> VVGGTEAQRNSWPSQISLQYRSGSSWAHTCGGTLIRQNWVMTAAHCVDRELTFRVVVGEHNLNQNNGTEQYVGVQKIVVHPYWNTDDVAAGYDIALLRLAQSVTLNSYVQLG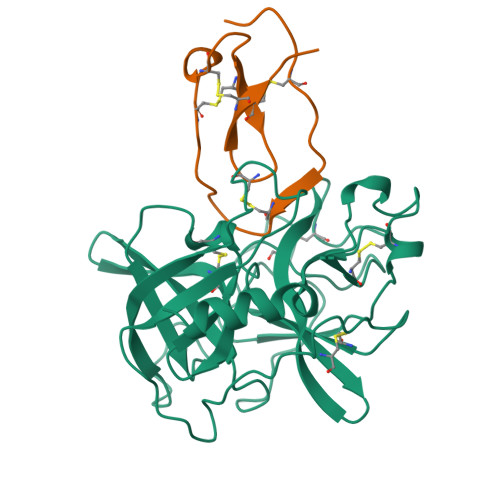VLPRAGTILANNSPCYITGWGLTRTNGQLAQTLQQAYLPTVDYAICSSSSYWGSTVKNSMVCAGGDGVRSGCQGDSGGPLHCLVNGQYAVHGVTSFVSRLGCNVTRKPTVFTRVSAYISWINNVIASN;> AQEPVKGPVSTKPGSCPIILIRCAMLNPPNRCLKDTDCPGIKKCCEGSCGMACFVPQ S-[5-[(E)-2-phenylethenyl]-1,3,4-oxadiazol-2-yl] 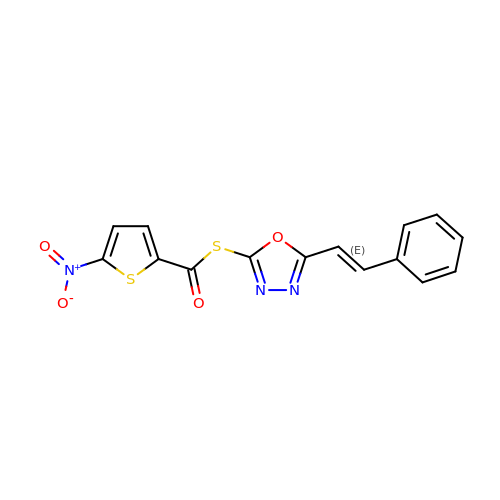5-nitrothiophene-2-carbothioate | C15 H9 N3 O4 S2 | QDBPRPJMSSSIEX-SOFGYWHQSA-N>MVSEYIDSELKRLEDYALRRVKGIPNNRRLWVLTCMDERVHIEQSLGIQPDDAHIYRNAGGIVTDDAIRSASLTTNFFGTKEIIVVTHTDCGMLRFTGEEVAKYFISKGIKPTEVQLD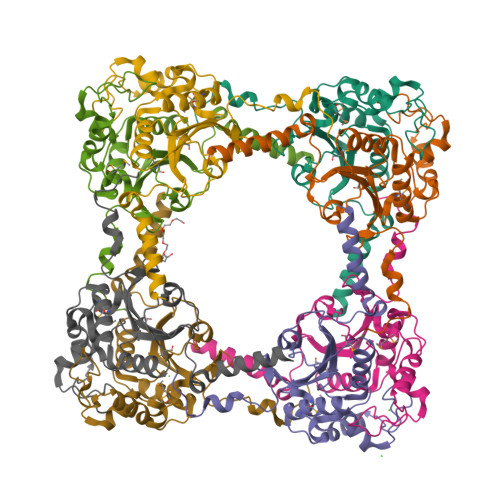PLLPAFRISSEEDFIKWFKFYEDLGVKSPDEMALKGVEILRNHPLIPKDVRITGYVYEVETHRLRKPNQIIYNETSKFEHGTIVKE[16x]>[6x]MKRVLVTLGAVAALATGAVAGGGAHWGYSGSIGPEHWGDLSPEYLMCKIGKNQSPIDINSADAVK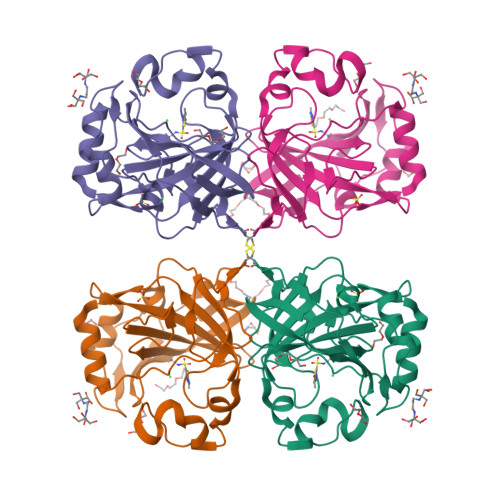ACLAPVSVYYVSDAKYVVNNGHTIKVVMGGRGYVVVDGKRFYLKQFHFHAPSEHTVNGKHYPFEAHFVHLDKNGNITVLGVFFKVGKENPELEKVWRVMPEEPGQKRHLTARIDPEKLLPENRDYYRYSGSLTTPPCSEGVRWIVFKEPVEMSREQLEKFRKVMGFDNNRPVQPLNARKVMK> MTHDNKLQVEAIKRGTVIDAIPAQIGFKLLSLFKLTETDQRITIGLN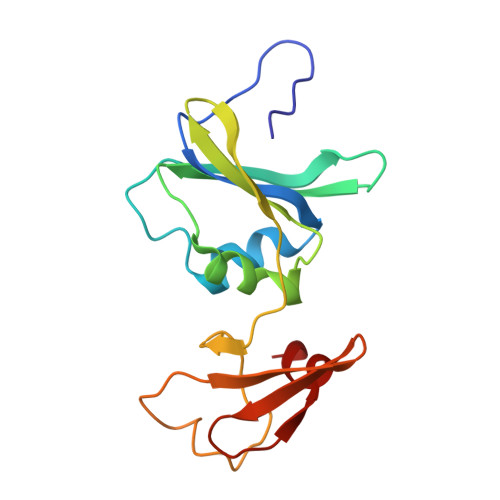LPSGEMGRKDLIKIENTFLSEDQVDQLALYAPQATVNRIDNYEVVGKSRPSLPERIDNVLVCPNSNCISHAEPVSSSFAVRKRANDIALKCKYCEKEFSHNVVLAN> MQLTPTFYDNSCPNVSNIVRDTIVNELRSDPR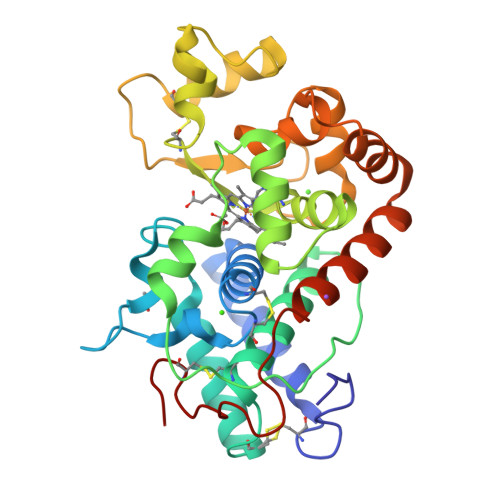IAASILRLHFHDCFVNGCDASILLDNTTSFRTEKDAFGNANSARGFPVIDRMKAAVESACPRTVSCADLLTIAAQQSVTLAGGPSWRVPLGRRDSLQAFLDLANANLPGPFFTLPQLKDSFRNVGLNRSSDLVALSGGHTFGKNQCRFIMDRLYNFSNTGLPDPTLNTTYLQTLRGLCPLNGNLSALVDFDLRTPTIFDNKYYVNLEEQKGLIQSDQELFSSPNATDTIPLVRSFANSTQTFFNAFVEAMDRMGNITPLTGTQGQIRLNCRVVNSNS> MGEQPIFSTRAHVFQIDPNTKKNWVPTSKHAVTVSYFYDSTRNVYRIISLDGSKAIINSTITPNMTFTKTSQKFGQWADSRANTVYGLGFSSEHHLSKFAEKFQEFKEAARLAKEKSQ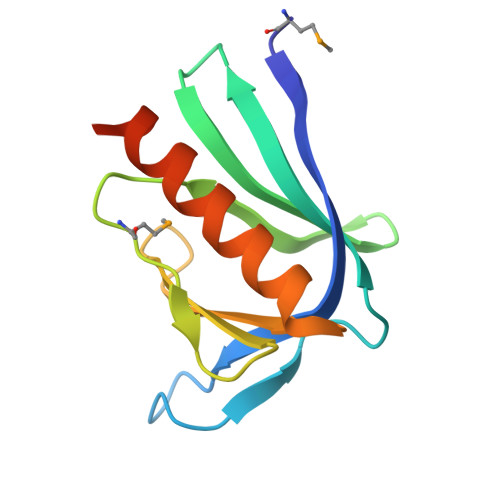EK> GAPPAPALRIDYPKALQILTEGGTHMVCTGRTHTDRLCRFKWLCYSSEA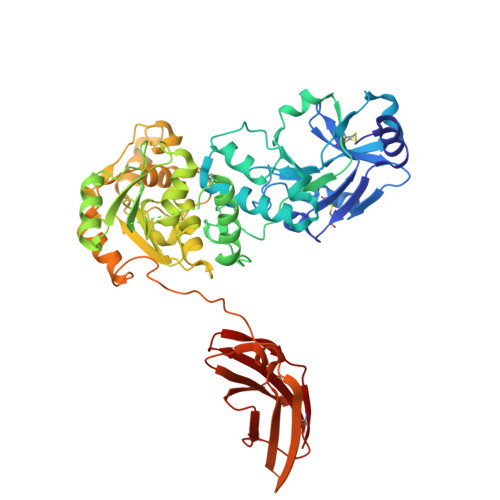EEFIFFHGNASVMLPSLGSRRFQPALLDLSTVEDHNTQYFNFVELPAAALRFMPKPVFVPDVALIANRFNPDNLMHVFHDDLLPLFYTLRQFPGLAREARLFFMEGWGEGAHFDLYKLLSPKQPLLRAQLKALGRLLCFSHAFVGLSKVTTWYQYGFVQPQGPKANILVSGNEIRQFAHFLMEKLNVSQAGGPLGEEYILVFSRTQNRLILNEAELLLALAQEFQMKTVTVSLEDHAFADVVRLVSNASMLVSMHGAQLVTALFLPRGAAVVELFPYAVNPDHYTPYKTLATLPGMDLQYIAWQNTMPENTVTHPERPWDQGGIAHLDRAEQARILQSREVPRHLCCRNPEWLFRIYQDTKVDIPSLIQTIRRVVKGHPGPRKQKWTVSLYPGKVREARCQASVQGASEARLSVSWQIPWNLKYLKVREVKYEVWLQEQGENTYVPYMLALQNHTFTENIKPFTTYLVWIRCIFNKTLLGPFADVLVCST>[19x]QARILEADAEILR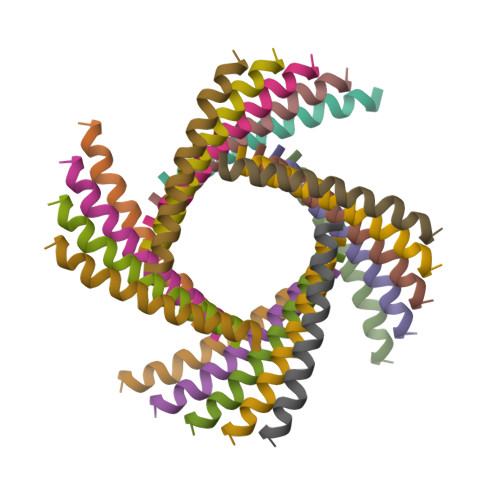AYARILEAHAEILRAQ> WSHPQFEKGATGRTTIAIDPVTRIEGHLKAEVVVENGKVVDARLSGGMYRGFETILRGRDPRDASQIVQRICGVCPTAHSTASVLALDEAFGAKVPNNGRITRNLIFGANYLQSHILHFYHLSAQDFVQGPDTAPFVPRFPKSDLRLSKELNK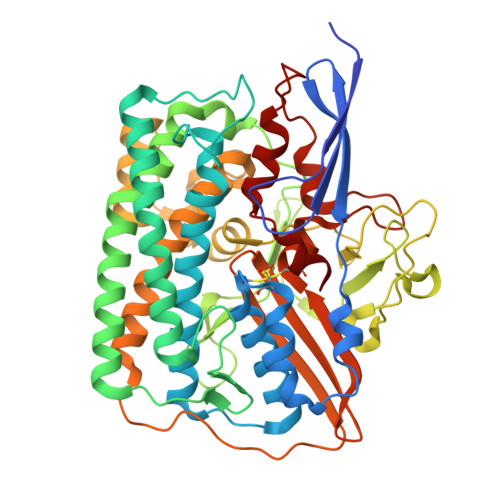AGVDQYIEALEVRRICHEMVALFGGRMPHVQGQVVGGATEIPTKEKLVEYAARFKKVRDFVEQKYVPVVYTIGSKYKDMFKVGQGFKAALCVGAFPLDNSGKKHLFMPGVYAKGKDMPFDPSKIKEYVKYSWFAEETTGLNYKEGKTIPAPDKAGAYSFVKAPRYDGLSLEVGPLARMWVNNPELSPVGKKLLKDLFGISAKKFRDLGEEAAFSLMGRHVARAEETYYMLGAIEGWLKEIKAGEDTVVMPAVPASAEGTGFTEAPRGSLLHYVKVKDSKIDNYQIVSASLWNCNPRDDMGQRGAVEEALIGIPVDDIQNPVNVARLIRAFDPULSCAVH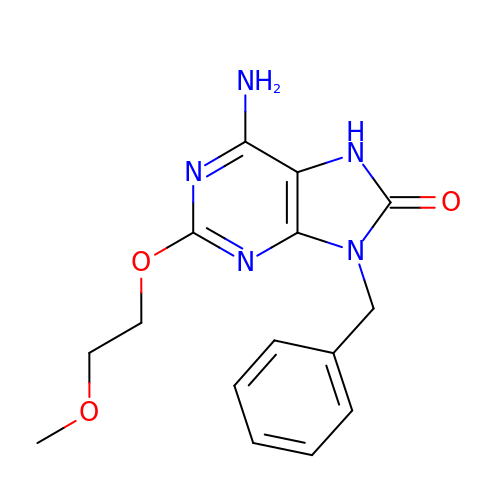6-azanyl-2-(2-methoxyethoxy)-9-(phenylmethyl)-7H-purin-8-one | C15 H17 N5 O3 | YYCDGEZXHXHLGW-UHFFFAOYSA-N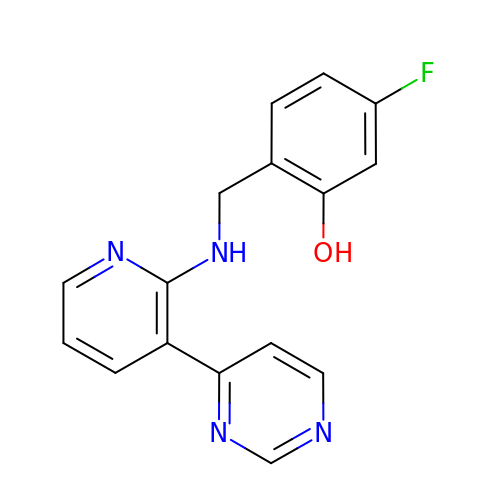5-fluoro-2-({[(3M)-3-(pyrimidin-4-yl)pyridin-2-yl]amino}methyl)phenol | C16 H13 F N4 O | GEXFOIODJDMVND-UHFFFAOYSA-N>MLSPKAATLAERSAGLAFSLYQAMAKDQAVENILLSPVVVASSLGLVSLGGKATTASQAKAVLSAEQLRDEEVHAGLGELLRSLSNSTARNVTWKLGSRLYGPSSVSFAEDFVRSSKQHYNCEHSKINFRDKRSALQSINEWAAQTTDGKLPEVTKDVERTDGALLVNAMFFKPHWDEKFHHKMVDNRGFMVTRSYTVGVTMMHRTGLYNYYDDEKEKLQIVEMPLAHKLSSLIILMPHHVEPLERLEKLLTKEQLKIWMGKMQKKAVAISLPKGVVEVTHDLQKHLAGLGLTEAIDKNKADLSRMSGKKDLYLASVFHATAFEWDTEGNPFDQDIYGREELRSPKLFYADHPFIFLVRDTQSGSLLFIGRLVRPKGDKMRDELLEHHHHH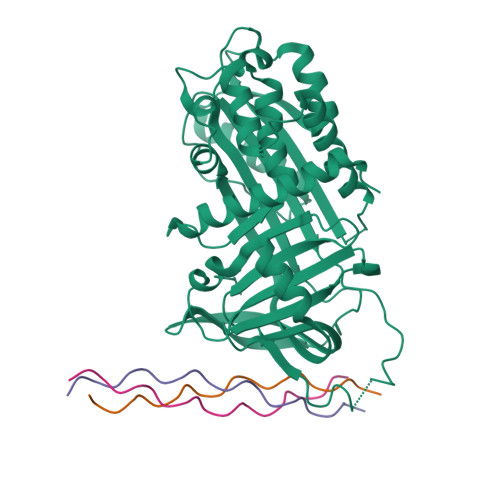H[2x];>[6x]XPPGPPGPPGPRGLPGPPGPPG(3S,6S)-3-{[4-(hydroxymethoxy)phenyl]methyl}-6-[(4-hydroxyphenyl)methyl]piperazine-2,5-dione | C19 H20 N2 O5 | 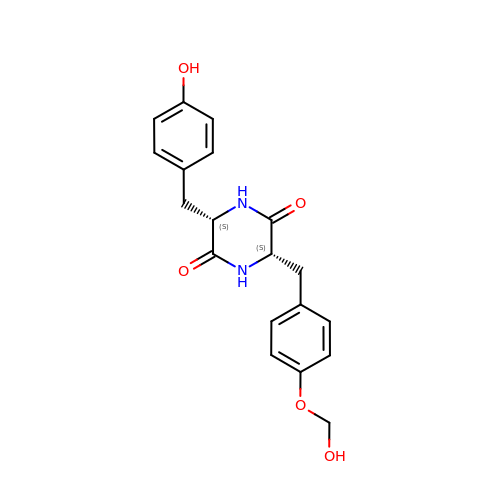XYLVFIWANSQWOX-IRXDYDNUSA-N> GSHMSKKILIVESDTALSATLRSALEGRGFTVDETTDGKGSVEQIRRDRPDLVVLAVDLSAGQNGYLICGKLKKDDDLKNVPIVIIGNPDGFAQHRKLKAHADEAVAKPVDADQLV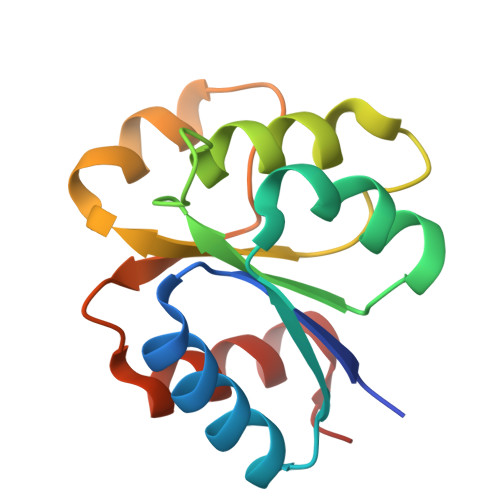ERAGALIGFPE>[3x]NIPDLAKKLGSSYALGAAIDQTALDPKDPHSELLTKHFNSITAGNFMKMDAMQPTEGKFVWSEADKLVNFAAANNMQVRGHTLLWHSQVP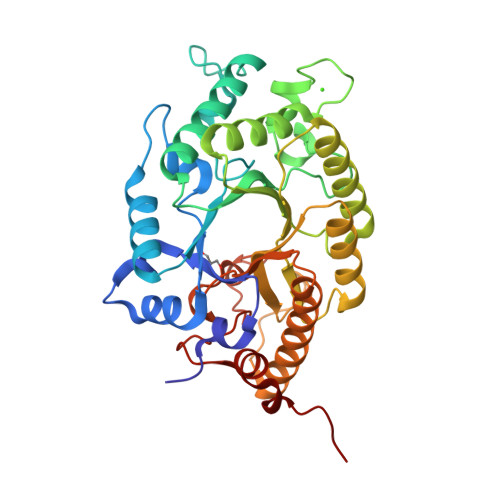DWFFTDPNDPSKPATREQLMQRMKTHIQTIVSRYKGKVHTWDVVNEVISDGGGLRNQASGSKWRDIIGDVDGDGDDSDYIELAFRYAREADPDAVLVINDYGIEGSVSKMNDMVKLVEKLLAKGTPIDAIGFQMHVSMYGPDIKQIREAFNRAAALGVHIQVTELDMSIYSGNSEQEKPVTDEMMLEQAYRYRALFDLFKEFDDRGVMDSVTLWGLADDGTWLDDFPVKGRKDAPLLFDRKLKAKPAYWALVDPSTLPVYRN>GMEVIESKWYKKDGASSASIDDVEKLLNTTLPKQYKSFLLWSNGGEGKLGDNYIYIWAIEDVIAYNHDYGIQKYLQKEYWAFGMDGDIGYILHLSDNSIYRVDLGDLDITSIKYIAPSFDDFLGKAIYLNF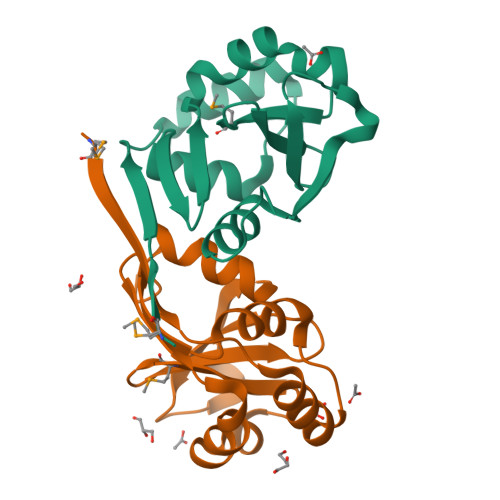NKLQNVANNNLTT[2x]>GSHMTPPHNYLAVIKVVGIGGGGVNAVNRMIEQGLKGVEFIAINTDAQALLMSDADVKLDVGRDSTRGLGAGADPEVGRKAAEDAKDEIEELLRGADMVFVTAGEGGGTGTGGAPVVASIARKLGALTVGVVTRPFSFEGKRRSNQAENGIAALRESCDTLIVIPNDRLLQMGDAAVSLMDAFRSADEVLLNGVQGITDLITTPGLINVDFADVKGIMSGAGTALMGIGSARGEGRSLKAAEIAINSPLLEASMEGAQGVLMSIAGGSDLGLFEINEAASLVQDAAHPDANIIFGTVIDDSLGDEVRVTVIAAGFDVSGPGRKPVMGETGGAHRIESAKAGKLTSTLFEPVDAVSVPLHTNGATLSI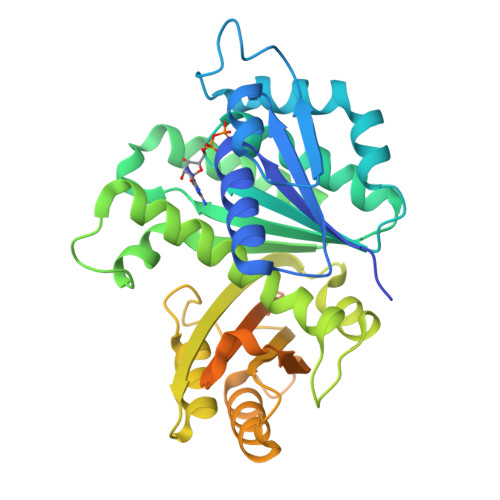GGDDDDVDVPPFMRR[3x]methyl 1-seleno-alpha-L-fucopyranoside | 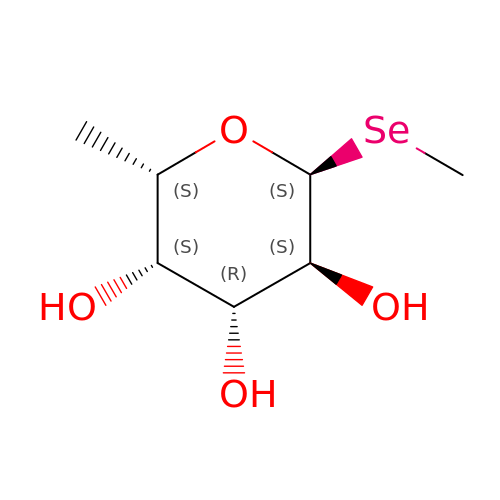C7 H14 O4 Se | VHTNTJQSKJZERS-XUVCUMPTSA-N> GHMAKQYDSVECPFCDEVSKYEKLAKIGQGTFGEVFKARHRKTGQKVALKKVLMENEKEGFPITALREIKILQLLKHENVVNLIEICRTKASPYNRCKGSIYLVFDFCEHDLAGLLSNVLVKFTLSEIKRVMQMLLNGLYYIHRNKILHRDMKAANVLITRDGVLKLADFGLARAFSLAKNSQPNRYTNRVVTLWYRPPELLLGERDYGPPIDLWGAGCIMAEMWTRSPIMQGNTEQHQLALISQLCGSITPEVWPNVDNYELYEK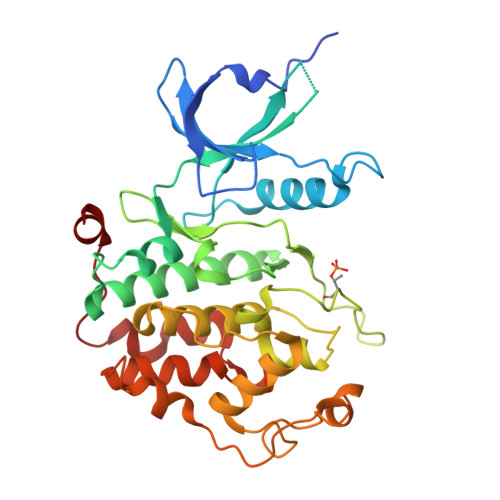LELVKGQKRKVKDRLKAYVRDPYALDLIDKLLVLDPAQRIDSDDALNHDFFWSDPMPSDLKGMLST> NLQNIIYNPVIPFVGTIPDQLDPGTLIVIRGHVPSDADRFQVDLQNGSSMKPRADVAFHFNP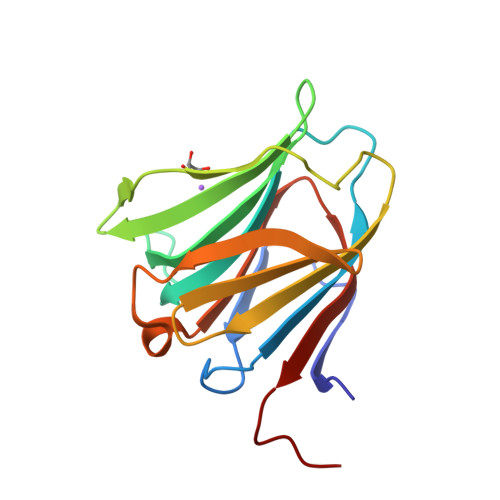RFKRAGCIVCNTLINEKWGREEITYDTPFKREKSFEIVIMVLKDKFQVAVNGKHTLLYGHRIGPEKIDTLGIYGKVNIHSIGFSFSSDLQ> GSTGPLGSMGSVLSSGQPTEEQLKMA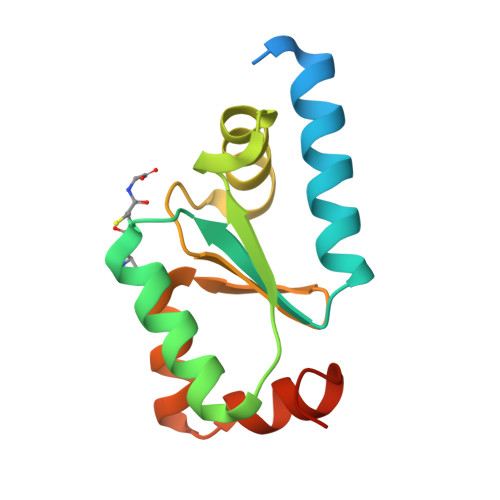LQKAQQLVNSNPLVVFSKTYCGYCSRVKKLFDQLGARYQTIELDQESDGDAIQAALLQWTGQRTVPNVFIGGKHIGGCDSVMEKHRDGKLVPMLTECGAIAIESTA> MEQLTKNQAVATSQEAVQNQNEPQLRDENAHNDKSVHGVLNPTYQAGLRR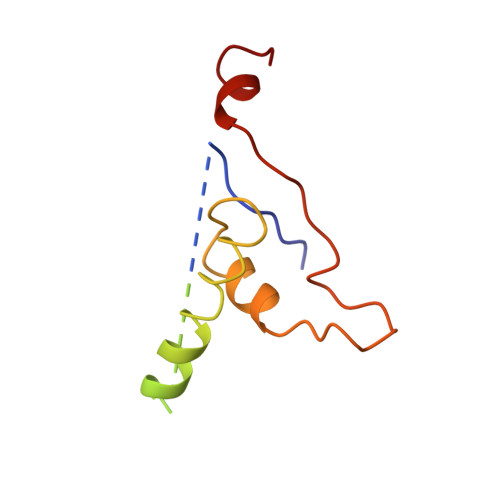DAVQPDIEAERKKRDEIEAGKSYCSRRFGGATCDDKSAQIYARFDKNDWRIQPAEFYRFHDAEVNTFGYF2-FUROIC ACID | C5 H4 O3 | 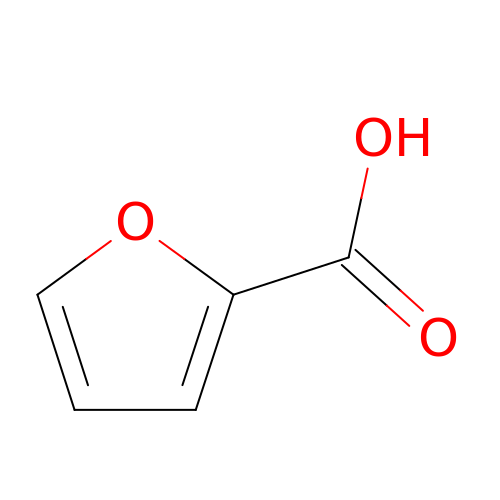SMNDYUVBFMFKNZ-UHFFFAOYSA-N> ENLACDEV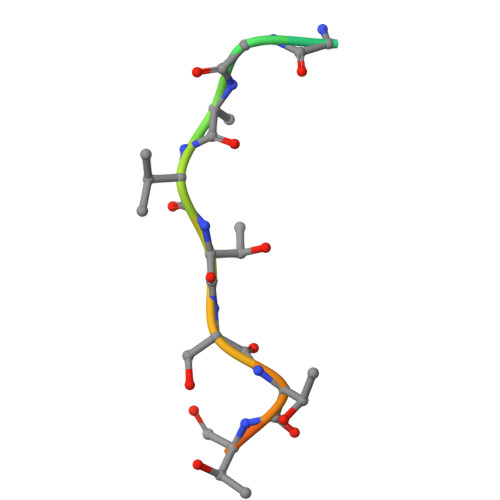TSTTSSST> GRLFKITACVPSQTRIRTQRELQNTYFTKLVPYENWFREQQ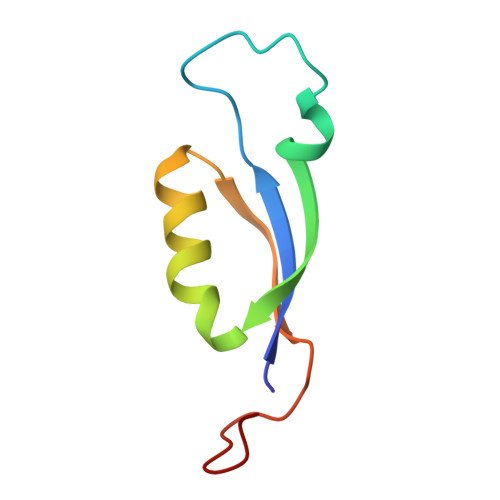RIQKMGGKIVKVELATGKQGINTGLA>MSTDKTDVKMGVLRIYLDGAYGIGKTTAAEEFLHHFAITPNRILLIGEPLSYWRNLAGEDAICGIYGTQTRRLNGDVSPEDAQRLTAHFQSLFCSPHAIMHAKISALMDTSTSDLVQVNKEPYKIMLSDRHPIASTICFPLSRYLVGDMSPAALPGLLFTLPAEPPGTNLVVCTVSLPSHLSRVSKRARPGETVNLPFVMVLRNVYIMLINTIIFLKTNNWHAGWNTLSFCNDVFKQKLQKSECIKLREVPGIEDTLFAVLKLPEL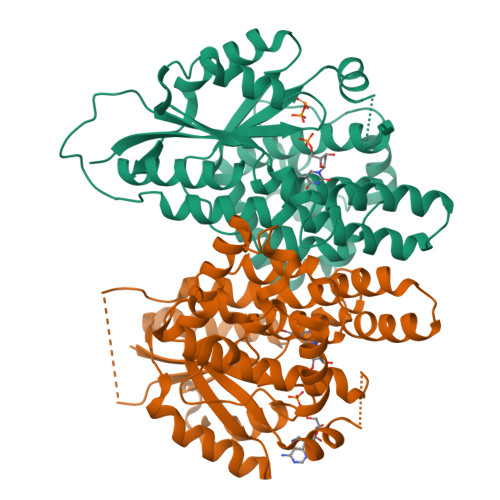CGEFGNILPLWAWGMETLSNCLRSMSPFVLSLEQTPQHAAQELKTLLPQMTPANMSSGAWNILKELVNAVQDNTS[4x]>MGSSHHHHHSSGENLYFQGHMFAPAPALPVSDADPFALDVLQDPLPFQANLRDAGPVVYLRRYDVFALGRYEQVHAALTDWQSFQSAAGVGLSNFRYETPWRPPSILLEADPPHHDAPRAVLSKILGPRALQKLRAAWIQDAEALVDQLLANTTEFDAVTDLAAAFPLRVFPDAVGIPDAGRENLLPYGDHAFNAFGPANGLVEKGAPRVAELSGWVNAQCARDALTGDGFGAQIWAAADRGDITYEQAPLVVRSLLTAGVDTTVNGLAAVLYAFATHPDQWARLRENRTLARTAFDEAVRWESPVQTFFRTATRDTEIGGATIPDGKKILMFLGAANRDPRRWENPEVFDLGRNPSGHVGYGMGIHQCVGQHVARLESEALLTALASRVHSLEIAGPVHRHLNNTLRSWESVPVKVRLP[2x]

We recently identified PbdA, a P450 from Rhodococcus jostii RHA1, and PbdB, its cognate reductase, which catalyze the O-demethylation of para-methoxylated benzoates (p-MBAs) to initiate growth of RHA1 on these compounds. PbdA is a member of the CYP199A family, which appears to have evolved to O-demethylate p-MBAs. Atomic-resolution structures of PbdA in complex with p-MBA, p-ethylbenzoate, and veratrate revealed a cluster of three residues that form hydrogen bonds with the substrates’ carboxylate: Ser87, Ser237, and Arg84. Similar to the substrate-bound structures of CYP199A2 and CYP1994, all three structures were in a closed conformation, with the F and G helices occluding the substrate access channel.

PbdA had the highest affinity (Kd = 3.8 ± 0.6 μM) and apparent specificity (kcat/KM = 20,000 ± 3000 M-1 s-1) for p-MBA. PbdA bound p-MBA, veratrate, and isovanillate with the highest affinity for p-MBA. Moreover, the binding of p-MBA resulted in a near 100% transition of the heme iron to the high-spin form. The structure of the three complexes are very similar to each other (RMSD of 0.176–0.683 Å of αC) as well as to the other CYP199As (e.g., RMSD of PbdA·p-MBA with CYP199A4·p-MBA and CYP199A2·p-MBA is 0.989 Å and 0.883 Å, respectively). Substrate orientation is maintained by four hydrogen bonds to the carboxylate, one from ordered water and three from active site residues Arg84, Ser87, and Ser237. The ordered water is localized by hydrogen bonding by heteroatoms in Arg236 and Ser237 side chains. The aromatic ring of the substrate is stabilized by hydrophobic interactions with Leu90 and Ala241. Residues Phe173, Phe176, Phe291, Ala241, Thr245, and Val288 form a hydrophobic pocket for the aromatic ligand. The high affinity and specificity of PbdA for p-MBA is consistent with what has been reported for two members of CYP199A subfamily, A2, and A4, (18).>GSTSDVANLANEKEEL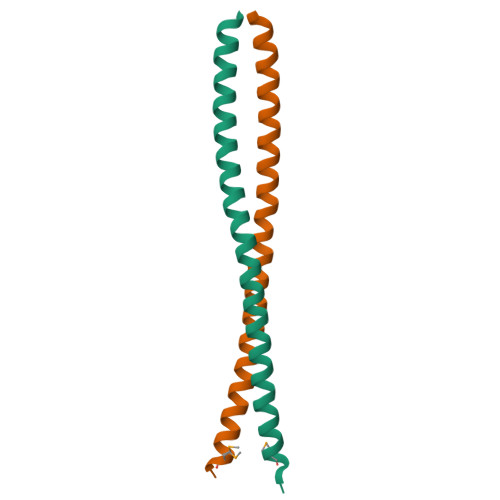NNKLKEAQEQLSRLKDEEISAAAIKAQFEKQLLTERTLKTQAVNKLAEIMNRKEP[2x]>GSWFFKNLSRKDAERQLLAPGNTHGSFLIRESESTAGSFSLSVRDFDQNQGEVVKHYKIRNLDNGGFYISPRITFPGLHELVRHYTNASDGLCTRLSR[2x];>XQFEEIP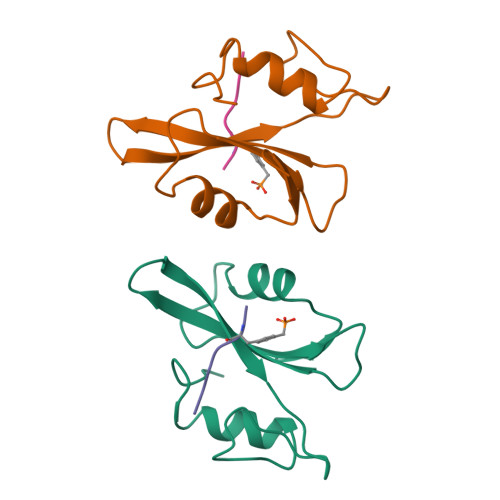[2x]>[2x]MTLTQEQRLVLDAVRRVAREVLYPLAPEYDRKAEYPWPQLKALAELGLLGMTTPEEWGGVGLDSVTWALALEELAAADPSVAVIVSVTSGLPQYMLLRFGSEAQKRRYLVPLARGEWIGAFCLTEPQAGSDAKSLRAEARRVKG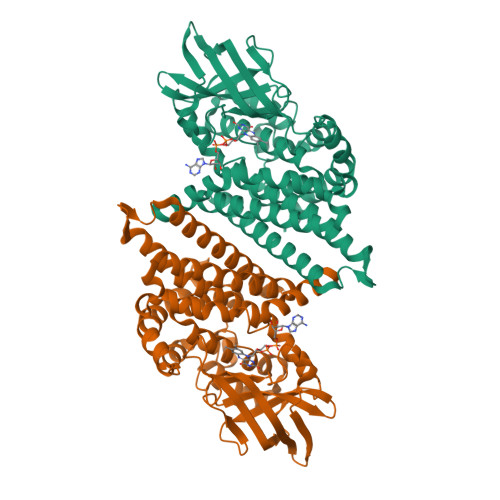GFVLNGVKSWITSAGHAHLYVVMARTEKGISAFLVEKGTPGLSFGRPEEKMGLHAAHTAEVRLEEVFVPEENLLGEEGRGLAYALAGLDSGRVGVAAQAVGIARGAFEIAKAYAEEREQFGKKLKEHQAIAFKIADMHVKIAAARALVLEAARKKDRGERFTLEASAAKLFASAAAVEVTREAVQVLGGYGYHRDYRVERYYRDAKVTEIYEGTSEIQRLVIARELYR>LPIDLRGKRAFIAGIADDNGYGWAVAKSLAAAGAEILVGTWVPALNIFETSLRRGKFDQSRVLPDGSLMEIKKVYPLDAVFDNPEDVPEDVKANKRYAGSSNWTVQEAAECVRQDFGSIDILVHSLGNGPEVSKPLLETSRKGYLAAISASSYSFVSLLSHFLPIMNPGGASISLTYIASERIIPGYGGGMSSAKAALESDTRVLAFEAGRKQNIRVNTISAGPLGSRAAKAIGFIDTMI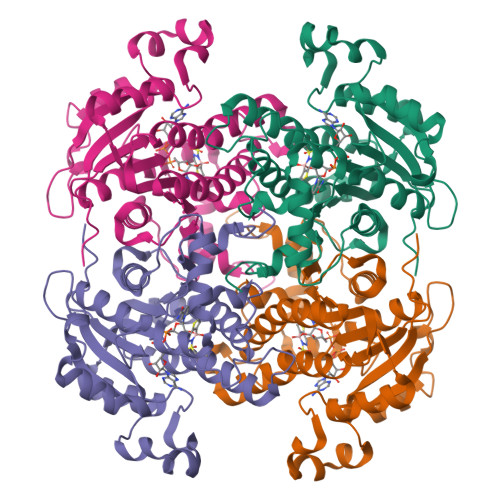EYSYNNAPIQKTLTADEVGNAAAFLVSPLASAITGATIYVDNGLNSMGVALDSPVF[2x]> MASMTGGQQMGRGSSGSPGVEQHTQAFLEALEQGGGKPLEQLSPKDARAVLTGAQASVKVDLSGIEVKERTIQANGQSIKLQVVRPANVKGELPVFMFFHGGGWVLGDFPTHQRLIRDLVVGSGAVAVYVDYTPSPESHYPTAINQ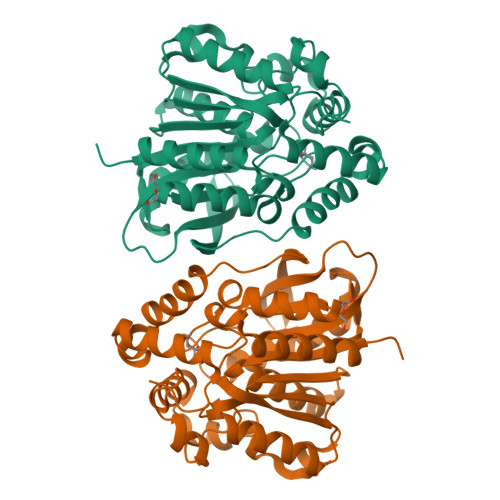AYAATQWVAEHGKEIGVDGKRLAVAGNSVGGNMAAVVALKAKEAGTPALRFQLLLWPVTDASFETASYKQFADGHFLTTGMMKWFWDNYTTDAKAREQIYASPLRASSEQLKGLPPALVQTAEFDVLRDEGEAYARKLNAAGVTVTSVRYNGMIHDYGLLNPLSQVPAVKAAMRQAGTELKVHLQLELEHHHHHH> MSLIDFHVHLDLYPDPVAVARACEERQLTVLSVTTTPAAWRGTLALAAGRPHVWTALGFHPEVVSERAADLPWFDRYLPETRFVGEVGLDGSPSLRGTWTQQFAVFQHILRRCEDHGGRILSIHSRRAESEVLNCLEANPRSGTPILHWYSGSVTELRRAISLGCWFSVGPTMVRTQKGAALIRSMPRDRVLTETDGPFLELDGQAALPWDVKSVVEGLSKIWQIPASEVERIVKENVSR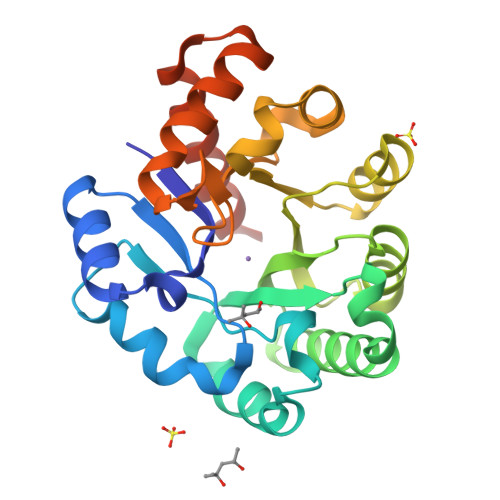LLGTVREGHHHHHH>[4x]MASMKVAVLPGDGIGPEVTEAALKVLRALDEAEGLGLAYEVFPFGGAAIDAFGEPFPEPTRKGVEEAEAVLLGSVGGPKWDGLPRKIRPETGLLSLRKSQDLFANLRPAKVFPGLERLSPLKEEIARGVDVLIVRELTGGIYFGEPRGMSEAEAWNTERYSKPEVERVARVAFEAARKRRKHVVSVDKANVL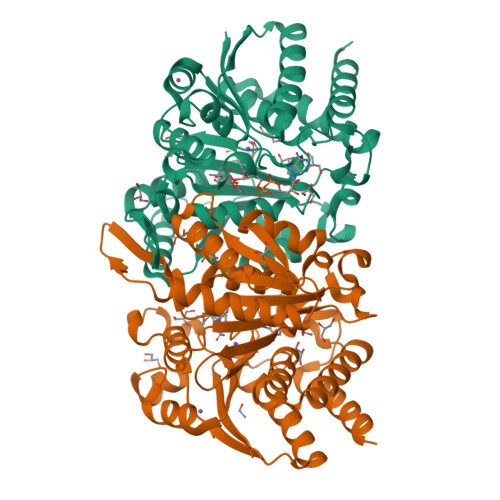EVGEFWRKTVEEVGRGYPDVALEHQYVDAMAMHLVRSPARFDVVVTGNIFGDILSDLASVLPGSLGLLPSASLGRGTPVFEPVHGSAPDIAGKGIANPTAAILSAAMMLEHAFGLVELARKVEDAVAKALLETPPPDLGGSAGTEAFTATVLRHLAAAALEHHHHHH> GSHMTTPSHLSDRYELGEILGFGGMSEVHLARDLRDHRDVAVKVLRADLARDPSFYLRFRREAQNAAALNHPAIVAVYDTGEAETPAGPLPYIVMEYVDGVTLRDIVHTEGPMTPKRAIEVIADACQALNFSHQNGIIHRDVKPANIMISATNAVKVMDFGIARAI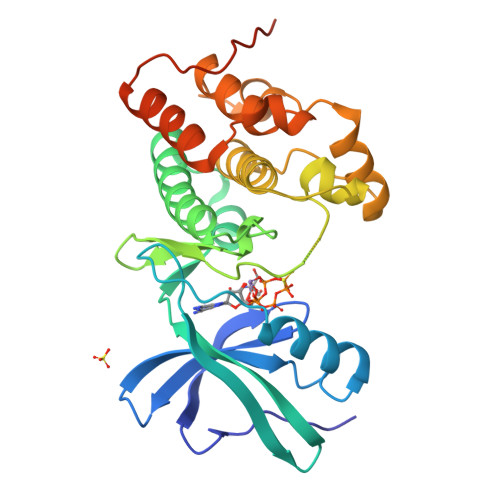ADSGNSVTQTAAVIGTAQYLSPEQARGDSVDARSDVYSLGCVLYEVLTGEPPFTGDSPVSVAYQHVREDPIPPSARHEGLSADLDAVVLKALAKNPENRYQTAAEMRADLVRVHNGEPPEAPKVLTDAERTSLLSSAAGNLSGPR3-(4-chlorophenyl)-5,6-dihydro-[1,3]thiazolo[2,3-b][1,3]thiazol-4-ium | C11 H9 Cl N S2 | 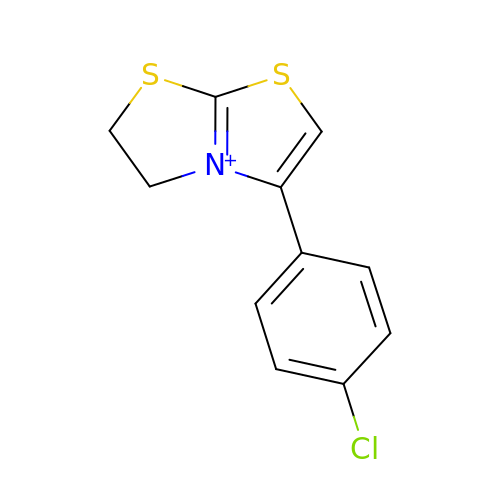XBGDFKDRBGVDQS-UHFFFAOYSA-N> MSAADFEAA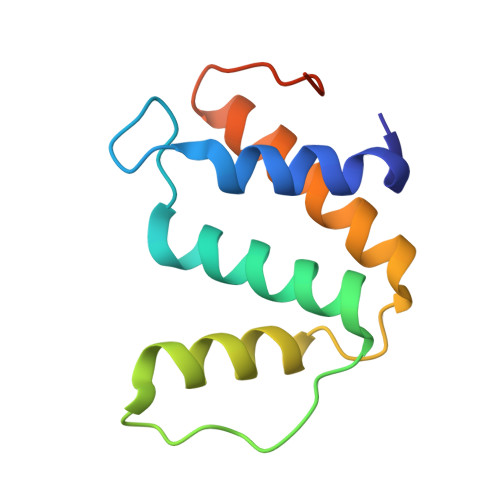VAYVRSLPKDGPVQLDNAAKLQFYSLYKQATEGDVTGSQPWAVQVEARAKWDAWNSCKGMKSEDAKAAYVRRLLTLLRSQGIQWKPGARVQSRL>[2x]SLNAIIIDDHPLAIAAIRNLLIKNDIEILAELTEGGSAVQRVETLKPDIVIIDVDIPGVNGIQVLETLRKRQYSGIIIIVSAKNDHFYGKHCADAGANGFVSKKEGMNNIIAAIEAAKNG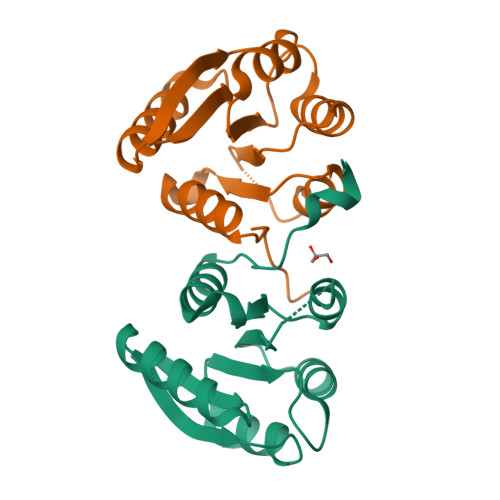YCYFPFSLNRFVGS>MADYKDDDDKSGRMKFFSYILVYRRFLFVVFTVLVLLPLPIVLHTKEAECAYTLFVVATFWLTEALPLSVTALLPSLMLPMFGIMPSKKVASAYFKDFHLLLIGVICLATSIEKWNLHKRIALKMVMMVGVNPAWLTLGFMSSTAFLSMWLSN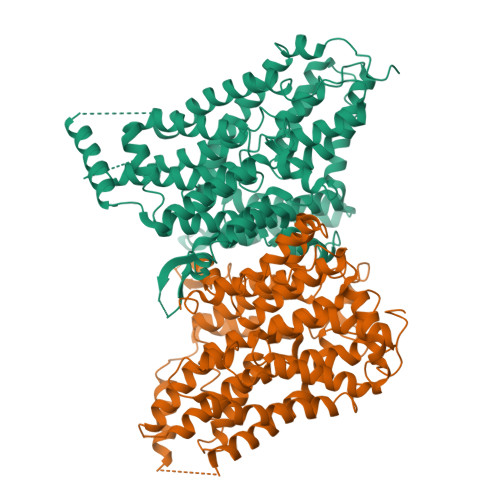TSTAAMVMPIAEAVVQQIINAEAEVEATQMTYFNGSTNHGLEIDESVNGHEINERKEKTKPVPGYNNDTGKISSKVELEKNSGMRTKYRTKKGHVTRKLTCLCIAYSSTIGGLTTITGTSTNLIFAEYFNTRYPDCRCLNFGSWFTFSFPAALIILLLSWIWLQWLFLGFNFKEMFKCGKTKTVQQKACAEVIKQEYQKLGPIRYQEIVTLVLFIIMALLWFSRDPGFVPGWSALFSEYPGFATDSTVALLIGLLFFLIPAKTLTKTTPTGEIVAFDYSPLITWKEFQSFMPWDIAILVGGGFALADGCEESGLSKWIGNKLSPLGSLPAWLIILISSLMVTSLTEVASNPATITLFLPILSPLAEAIHVNPLYILIPSTLCTSFAFLLPVANPPNAIVFSYGHLKVIDMVKAGLGVNIVGVAVVMLGICTWIVPMFDLYTYPSWAPAMSNETMP[2x]>[2x]MHNYSYSPGISLLLFILLANTLAIQAVVLPAHQQHLLHNDIADGLDKTALSVSGTQSRWTRSESNPTMRLSQNVKPCKSMDIRNMVSHFNQLENCTVIEGFLLIDLINDASPLNRSFPKLTEVTDYIIIYRVTGLHSLSKIFPNLSVIRGNKLFDGYALVVYSNFDLMDLGLHKLRSITRGGVRIEKNHKLCYDRTIDWLEILAENETQLVVLTENGKEKECRLSKCPGEIRIEEGHDTTAIEGELNASCQLHNNRRLCWNSKLCQTKCPEKCRNNCIDEHTCCSQDCLGGCVIDKNGNESCISCRNVSFNNICMDSC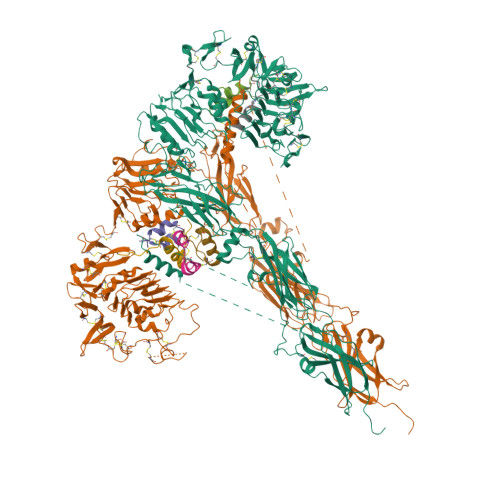PKGYYQFDSRCVTANECITLTKFETNSVYSGIPYNGQCITHCPTGYQKSENKRMCEPCPGGKCDKECSSGLIDSLERAREFHGCTIITGTEPLTISIKRESGAHVMDELKYGLAAVHKIQSSLMVHLTYGLKSLKFFQSLTEISGDPPMDADKYALYVLDNRDLDELWGPNQTVFIRKGGVFFHFNPKLCVSTINQLLPMLASKPKFFEKSDVGADSNGNRGSCGTAVLNVTLQSVGANSAMLNVTTKVEIGEPQKPSNATIVFKDPRAFIGFVFYHMIDPYGNSTKSSDDPCDDRWKVSSPEKSGVMVLSNLIPYTNYSYYVRTMAISSELTNAESDVKNFRTNPGRPSKVTEVVATAISDSKINVTWSYLDKPYGVLTRYFIKAKLINRPTRNNNRDYCTEPLVKAMENDLPATTPTKKISDPLAGDCKCVEGSKKTSSQEYDDRKVQAGMEFENALQNFIFVPNIRKSKNGSSDKSDGAEGAALDSNAIPNGGATNPSRRRRDVALEPELDDVEGSVLLRHVRSITDDTDAFFEKDDENTYKDEEDLSSNKQFYEVFAKELPPNQTHFVFEKLRHFTRYAIFVVACREEIPSEKLRDTSFKKSLCSDYDTVFQTTKRKKFADIVMDLKVDLEHANNTESPVRVRWTPPVDPNGEIVTYEVAYKLQKPDQVEEKKCIPAADFNQTAGYLIKLNEGLYSFRVRANSIAGYGDFTEVEHIKVEPPPSYAKDEVLFQGPSRSAWSHPQFEK;>DFRGVVDSCCRNSCSFSTLRAYCDS[3x];>NSLRACGPALMDMLRVACPNGFNSMFAK[3x]> GMTEAFPALVRQDDARYAITVGPDLAVGPPGHAYLFGGASMALALDVAAETVGRPVVQGSLQFVSFTPLGSVLDLTVEVLQSGRTLAQARVAGTVDGRLVFHSGISLGMREGFSARQWALAPPVPQPDNCPPCTTLPAQDDNARYLEGIEVREAGGPEVPSGRTRLWLRRKDG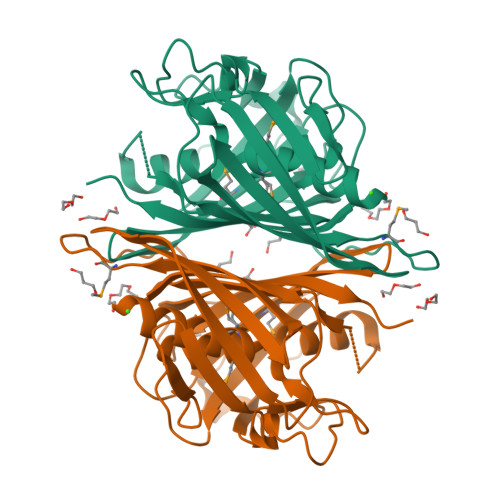APLDAASLAMFADFLPIALGRATGCSGGGNSLDNSLRITGAAAPGWCLCDMIIPSSASGFAQGQVTLWDQSGRLLATGAQSLLLKG The gene cluster containing the thal gene also encodes the flavin reductase ThdF. Hence, ThdF might provide reduced FADH2 for Thal in S. albogriseolus. In contrast, our steady-state kinetics showed that flavin reduction in ThdF follows an ordered sequential mechanism, with FAD binding as the first substrate followed by NADH and the respective products being released in reverse order.

The crystallization trials of ThdF in the presence of elastase resulted in two well-diffracting crystal forms (space groups: form 1: P212121; form 2: P21) of different packing with a resolution of 1.14 Å and 1.31 Å. Surprisingly, in both crystal forms, two FADs with very well-defined electron density were visible per ThdF molecule. The FAD closer to the dimer interface is stacked, bringing the adenine base and the isoalloxazine ring into close proximity. The stretched flavin forms 14 polar contacts to surrounding amino acids. The adenosine is flexible and adopts a flipped conformation in chain A of crystal form 1, suggesting that FMN should be able to bind almost as well as FAD. In ThdF, the two isoalloxazine rings are in parallel planes but orthogonal with ring III (two carbonyl moieties) of the stretched FAD (yellow carbon atoms) and ring I (two methyl groups) of the stacked FAD (wheat carbon atoms) being opposite of each other. This means that the central rings (ring II) are not directly above each other, which results in the two N5 atoms being relatively far apart (6.7 Å). The stacked FAD bound in the NADH binding site in two of our structures most likely does not represent a functional state. We assume that the unphysiologically low salt concentration during crystallization may favor the presumably nonphysiological state with two FADs per ThdF protomer.

>[4x]GAMAGAAGGVTTEQQHYRDLMSAFPTGIAVVTSLDAQGVPRGMTCSSVTSATLSPPTLLVCLRNGSATLDAVSATRGFAVNLLHDGGRHAAEVFSGPDPNRFSRVQWKQCRSGLPWLSKDAFAVAECRVSGTQEVGDHTVVFGEVARIAQTDGTPLLYGLRSFAAWPLPSESARQGSEAAPRGSEPAYGARSSRG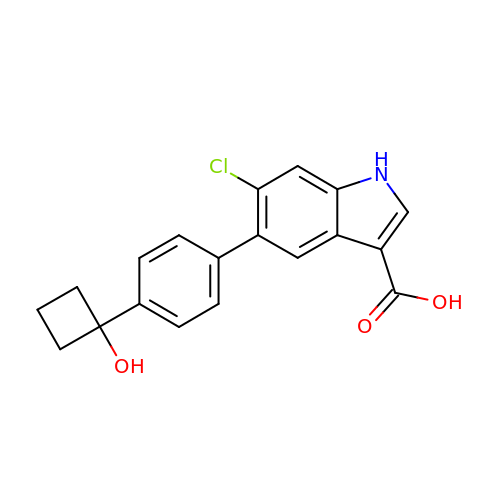6-chloranyl-5-[4-(1-oxidanylcyclobutyl)phenyl]-1~{H}-indole-3-carboxylic acid | C19 H16 Cl N O3 | FHQXLWCFSUSXBF-UHFFFAOYSA-N>MQSTPLLQIQPHFHVEVIEPKQVYLLGEQANHALTGQLYCQILPLLNGQYTLEQIVEKLDGEVPPEYIDYVLERLAEKGYLTEAAPELSSEVAAFWSELGIAPPVAAEALRQPVTLTPVGNISEVTVAALTTALRDIGISVQTPTEAGSPTALNVVLTDDYLQPELAKINKQALESQQTWLLVKPVGSVLWLGPVFVPGKTGCWDCLAHRLRGNREVEASVLRQKQAQQQRNGQSGSVIGCLPTARATLPSTLQTGLQFAATEIAKWIVKYHVNATAPGTVFFPTLDGKIITLNHSILDLKSHILIKRSQCPTCGDPKILQHRGFEPLKLESRPKQFTSDGGHRGTTPEQTVQKYQHLISPVTGVVTELVRITDPANPLVHTYRAGHSFGSATSLRGLRNTLKHKSSGKGKTDSQSKASGLCEAVERYSGIFQGDEPRKRATLAELGDLAIHPEQCLCFSDGQYANRETLNEQATVAHDWIPQRFDASQAIEWTPVWSLTEQTHKYLPTALCYYHYPLPPEHRFARGDSNGNAAGNTLEEAILQGFMELVERDGVALWWYNRLRRPAVDLGSFNEPYFVQLQQFYRENDRDLWVLDLTADLGIPAFAGVSNRKTGSSERLILGFGAHLDPTIAILRAVTEVNQIGLELDKVPDENLKSDATDWLITEKLADHPYLLPDTTQPLKTA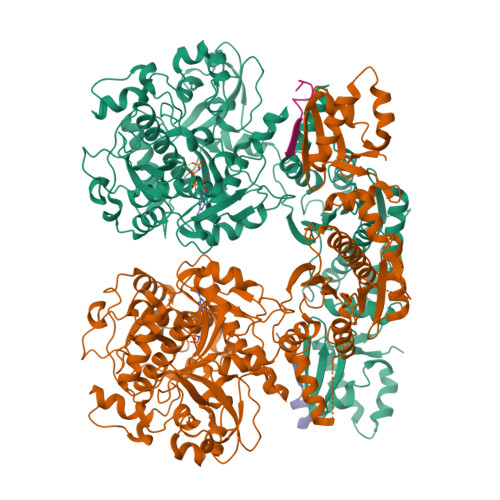QDYPKRWSDDIYTDVMTCVNIAQQAGLETLVIDQTRPDIGLNVVKVTVPGMRHFWSRFGEGRLYDVPVKLGWLDEPLTEAQMNPTPMPF[2x];>MDKKNILPQQGQPVIRLTAGQLSSQLAELSEEALGDAGLEASKITACITFAAYDGELEHHHHHH[2x]> MIFPKQYPIINFTTAGATVQSYTNFIRAVRGRLTTGADVRHEIPVLPNRVGLPINQRFILVELSNHAELSVTLALDMTNAAVVGYRAGNSAYFFHPDNQEDAEAITHLFTDVQNRYTFAFGGNYDRLEQLAGNLRENIELGNGPLEEAISALYYYSTGGTQLPTLARSFIICIQMISEAARFQYIEGEMRTRIRYNRRSAPDPSVITLENSWGRLSTAIQESNQGAFASPIQLQRRNGSKFSVYDVSILIPIIALMVYRC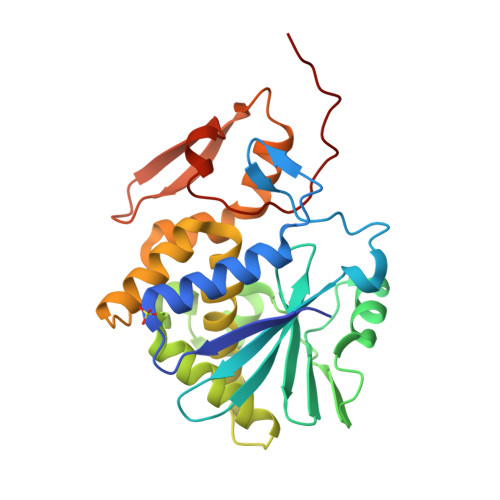APPPSSQF> GPSLDFALSLLRRNIRQVQTDQGHFTMLGVRDRLAILPRHSQPGKTIWVEHKLINVLDAVELVDEQGVNLELTLVTLDTNEKFRDVTKFIPETITGASDATLIINTEHMPSMFVPVGDVVQYGFLNLSGKPTHRT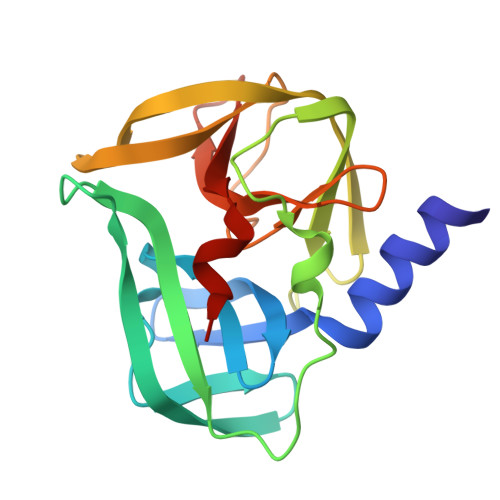MMYNFPTKAGQCGGVVTSVGKIIGIHIGGNGRQGFCAGLKRGYFASEQ>[2x]MSRLERLTSLNVVAGSDLRRTSIIGTIGPKTNNPETLVALRKAGLNIVRMNFSHGSYEYHKSVIDNARKSEELYPGRPLAIALDTKGPEIRTGTTTNDVDYPIPPNHEM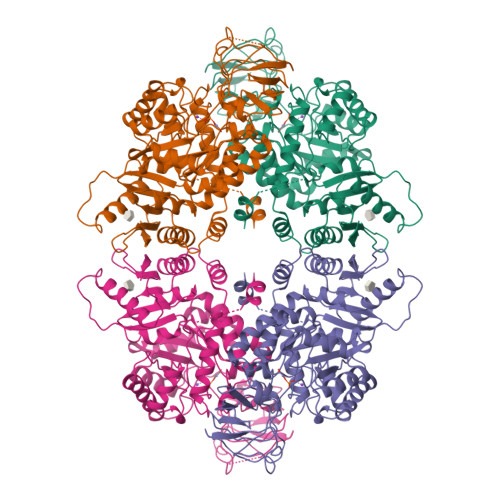IFTTDDKYAKACDDKIMYVDYKNITKVISAGRIIYVDDGVLSFQVLEVVDDKTLKVKALNAGKICSHKGVNLPGTDVDLPALSEKDKEDLRFGVKNGVHMVFASFIRTANDVLTIREVLGEQGKDVKIIVKIENQQGVNNFDEILKVTDGVMVARGDLGIEIPAPEVLAVQKKLIAKSNLAGKPVICATQMLESMTYNPRPTRAEVSDVGNAILDGADCVMLSGETAKGNYPINAVTTMAETAVIAEQAIAYLPNYDDMRNCTPKPTSTTETVAASAVAAVFEQKAKAIIVLSTSGTTPRLVSKYRPNCPIILVTRCPRAARFSHLYRGVFPFVFEKEPVSDWTDDVEARINFGIEKAKEFGILKKGDTYVSIQGFKAGAGHSNTLQVSTV> MAEIPKEMLRAQTNVILLNVLKQGDNYVYGIIKQVKEASNGEMELNEATLYTIFKRLEKDGIISSYWGDESQGGRRKYYRLTEIGHENMRLAFESWSRVDKIIENLEANKKSEAIK

LmrR belongs to the PadR-like family of transcriptional regulators (Pfam PF03551), which is named after a regulatory protein involved in the regulation of expression of phenolic acid decarboxylase (pad) genes. LmrR was shown to be a transcriptional repressor of lmrCD expression and an autoregulator of its own expression. LmrR forms a dimer with each monomer comprising a typical winged helix-turn-helix DNA binding domain and a C-terminal helix involved in dimerization. In between the two monomers is a large central pore that serves as the drug-binding site.

Riboflavin was identified as a ligand of LmrR by co-crystallization screening. The crystal structure of the riboflavin-bound LmrR complex (LmrR•RBF) was solved by molecular replacement and refined at 2.35 Å (see Table 1 for relevant crystallographic statistics). Extra density in the central drug-binding pore confirmed the presence of bound ligand, but docking of riboflavin was complicated by the occurrence of alternative binding modes. Different potential binding modes of RBF fitting the electron density were tested by short 200 ps molecular dynamics runs, resulting in the identification of two stable unique binding modes with similar predicted binding energy. These two binding modes of RBF are related by a ~180° flip of the heterocyclic isoalloxazine moiety relative to the ribityl side chain. The occupancy of each of the four binding modes in the crystal was estimated to be 0.25. The flat aromatic isoalloxazine ring of riboflavin slides into the center of the flat-shaped hydrophobic pore of the LmrR dimer, in between the indole rings of the central Trp96/Trp96’ pair, while the ribityl substituent protrudes towards the pore opening. Riboflavin recognition by LmrR is likely dominated by the aromatic stacking interactions of the Trp96/Trp96’ indole pair with the heterocylic aromatic core of riboflavin. Near the pore opening, Asp100 may contribute to the stabilization of the hydrophilic ribityl moiety of riboflavin, by the formation of hydrogen bonds, although the observed disorder of the ribityl moiety indicates that these interactions are quite weak. The dissociation constant (Kd) for binding of RBF to LmrR was determined as 0.26 ± 0.08 μM, using a fluorescence-based titration assay.>MTTKKFDEADKSNVEMYLIQAGVKQDAAATMGIWTAQELHRIKSQSYEEDYPVGSALRVFPVTTELSPTDKTFEYMTFDKVGTAQIIADYTDDLPLVDALGTSEFGKVFRLGNAYLISIDEIKAGQATGRPLSTRKASACQLAHDQLVNRLVFKGSAPHKIVSVFNHPNITKITSGKWIDVSTMKPETAEAELTQAIETIETITRGQHRATNILIPPSMRKVLAIRMPETTMSYLDYFKSQNSGIEIDSIAELEDIDGAGTKGVLVYEKNPMNMSIEIPEAFNMLPAQPKDLHFKVPCTSKCTGLTIYRPMTIVLITGV[7x];> MAYENLMLRPACPGNLSDTSTYNIDGACVAQGDIEFGSAVQVVGIVDGVKVVTALSDGGTPYGIAFRSQYEHLSGKILDGEVCNVVSHGRVWALTSLDEAPSLFSKLQFGSGGVVTGGSGYAGWTFAGGFVKHEDGYIIEVRVKQNAFIVPPPPPPVVLV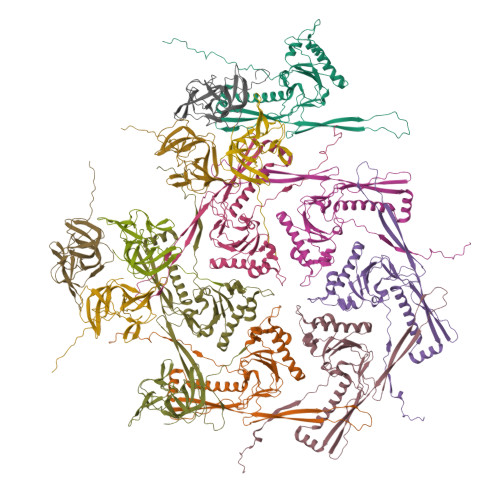ESATITTDKESPQPNNVTIQCVANALPANATDKTGKWSIDATNIATVNPDSGLVTPVGGEVVGDFNITWTANDASKTTATIAYRVEAVPTPEVDV;>[6x]MAQINASYQRDMAIALPGMVADTSKYNIDGACVVNEGDVLVGAAVQVVQAQAVDGHKLVKALTTGTTPYGVAIRSHWQTVNAQNQMIYEDGGAINVMTSGRVWMLSKSTEAPTFGSAVKLDVDGQEKSDGTIETTWTYAGGWTKYKDIQLVEVQLHQL>GPLTRRASVGSMSEKETNYVENLLTQLENELNEDNLPEDINTLLRKCSLNLVTVVSLPDMDVKPLLATIKRFLTSNVSYDSLNYDYLLDVVDKLVPMADFDDVLEVYSAEDLVKALRSEIDPLKVAACRVIENSQPKGLFATSNIIDILLDILFDEKVENDKLITAIEKALERLSTDELIRRRLFDNNLPYLVSVKGRMETVSFVRLIDFLTIEFQFISGPEFKDIIFCFTKEEILKSVEDILVFIELVNYYTKFLLEIRNQDKYWALRHVKKILPVFAQLFEDTENYPDVRAFSTNCLLQLFAEVSRIEEDEYSLFKTMDKDSLKIGSEAKLITEWLELINPQYLVKYHKDVVENYFHVSGYSIGMLRNLSADEECFNAIRNKFS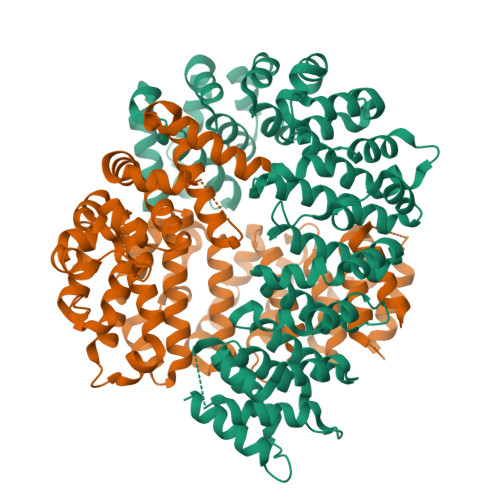AEIVLRLPYLEQMQVVETLTRYEYTSKFLLNEMPKVMGSLIGDGSAGAIIDLETVHYRNSALRNLLDKGEEKLSVWYEPLLREYSKAVNGKNYSTGSETKIADCR[2x]2,6-dichloro-N-{2-[(cyclopropylcarbonyl)amino]pyridin-4-yl}benzamide | C16 H13 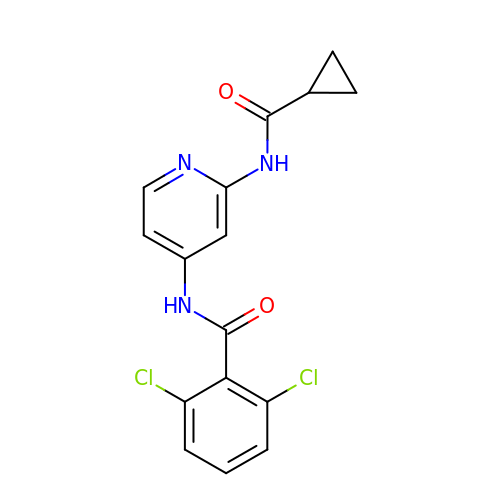Cl2 N3 O2 | IAFNAEGXTKTGHN-UHFFFAOYSA-N>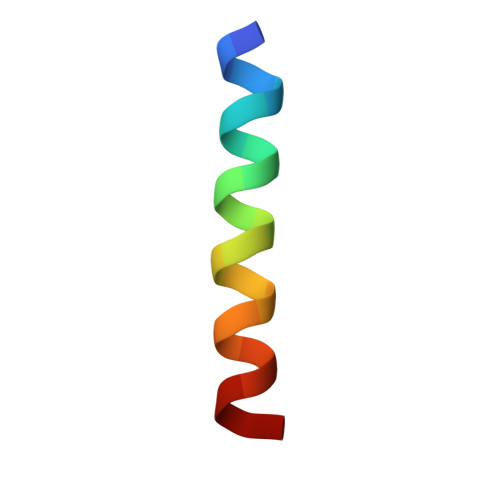 RPEIWAAQELRRIGDEFNAYYR> PAQDNSRFVIRDRNWHPKALTPDYKTSIARSPRQALVSIP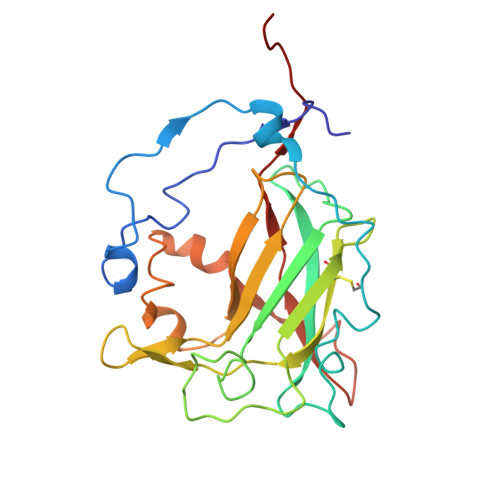QSISETTGPNFSHLGFGAHDHDLLLNFNNGGLPIGERIIVAGRVVDQYGKPVPNTLVEMWQANAGGRCRHKNDRYLAPLDPNFGGVGRCLTDSDGYYSFRTIKPGPYPWRNGPNDWRPAHIHFGISGPSIATKLITQLYFEGDPLIPMCPIVKSIANPEAVQQLIAKLDMNNANPMDCLAYRFDIVLRGQRKTHFENC> MSQRIIQPSASDQQFPGKSDGYEYTVGPKQAITSEASTTYIPSRIYSESLLFKRQEASLSAMAFLFQEMISQLHRTCKTAGDFETKLSDYGHNIGIRLLELLNFRASSSPSSLPRASAFLSQNESSSKLSNASNSPGMLANSSTAT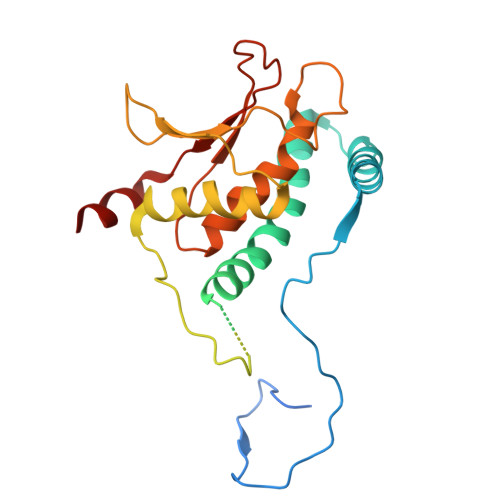SASANERLQEKQTESLSNYITKMRRRDLKILDILQFIHGTLWSYLFNHVSDDLVKSSERDNEYMIVDNFPTLTQFIPGENVSCEYFVCGIIKGFLFNAGFPCGVTAHRMPQGGHSQRTVYLIQFDRQVLDREGLRFG> GADNRELWKVLNVDLEKHDEFLAPVPAVYRELFLNRPNRPRAMAYFDAVVGDIHGIRVHELYNLKQEGKKVFATFCVYVPEEIINATGS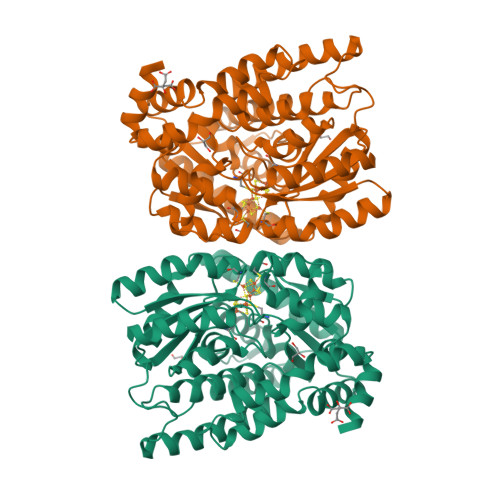ACIGLCGGAQYTVPAGETVLPRNLCPLIKSAMGFKIERICPYFQVADYVVGETTCDGKKKAWEILNEYIPVYVMELPQKKEERDRKFWEEEIKDFAQFVEEKTGVKLNAENLRAGIEKINKKRKALKRLSDLRKHNPAPIHGLDVLLINQLAFFDDPERFATKVNELCDELEERVAKGEGVVSKDAPRILITGTPQPIPHWKIHALIEGAGGVVVGEETCIGERYFKDLVEPAADVEGMLKNIAARSLKVNCACFTPNTGRLEDILSMVQKLQVDGVIHYSLQFCQPYGVESYLVGRELERRNIPFLKLESDFSEEDQGQLKTRIEAFLEMI>[4x]MAKPQVTILATGGTIAGSGESSVKSSYSAGAVTVDKLLAAVPAINDLATIKGEQISSIGSQEMTGKVWLKLAKRVNELLAQKETEAVIITHGTDTMEETAFFLNLTVKSQKPVVLVGAMRPGSSMSADGPMNLYNAVNVAINKASTNKGVVIVMNDEIHAAREATKLNTTAVNAFASPNTGKIGTVYYGKVEYFTQSVRPHTLASEFDISKIEELPRVDILYAHPDDTDVLVNAALQAGAKGIIHAGMGNGNPFPLTQNALEKAAKSGVVVARSSRVGSGSTTQEAEVDDKKLGFVATESLNPQKARVLLMLALTKTSDREAIQKIFSTY

By administering enzyme drugs called L-asparaginases, which act to quickly deplete Asn in the blood, this drug specifically impacts ALL cells, starving them to death while leaving normal cells largely intact. WoA, like most bacterial Type II L-asparaginases, is a tetramer built by a dimer-of-dimer with 330 residues per protomer. In our structures we observe that the overall fold of each protomer follows the general two-domain fold of bacterial type II L-asparaginases. We sought to clarify this question and to further explain the substrate discrimination, if there is any, between the two forms, by solving the crystal structures of both variants in complex with either the product Asp or L-glutamic acid (Glu).

Since all of the four structures presented here were solved in the presence of ligand, we expected the enzyme to adopt the closed N-terminal loop conformation in all structures. Indeed, this is what we observed in the WoA-P121 + Asp structure. For WoA-P121, soaking the crystal briefly in Asp solution was sufficient in closing the loop. To our knowledge, the WoA-S121 + Asp, WoA-S121 + Glu and WoA-P121 + Glu structures reported in this study represent the first L-asparaginase structures caught in its fully inactive/open state in the presence of product ligands, while the WoA-P121 + Asp structure is the first closed/active state of WoA reported so far. An identical Asp binding mode was also observed between the WoA-P121 + Asp and WoA-S121 + Asp structures, despite the former having the closed, and the latter the open, N-terminal loop conformation. In this comparison, WoA-P121 + Asp represents the closed/active state of the enzyme (pink), whereas WoA-P121 + Glu represents the open/inactive state (green). As the catalytically-relevant state is the one where the N-terminal loop is closed, to better understand how WoA-P121 would accommodate Glu in its closed state, we modelled into the open WoA-P121 + Glu structure the closed loop conformation as observed in the WoA-P121 + Asp structure. This modelling reveals that whereas Asp fits without strain into the closed active site, binding of the larger ligand Glu (Glu has an extra methylene group relative to Asp) seems to be incompatible with loop closure due to several steric clashes. When residue 121 is a proline, it strengthens the closed-conformation of Tyr27 ( ), which in turn stabilizes Thr14. Hence, the extra interaction provided by Pro121 (but not by Ser121) suffices to promote loop closure, rationalizing our observation of the WoA-P121 + Asp structure being in the closed conformation.> HMSPSPVPGSQNVPAPAVKKISQYACQRRTTLNNYNQLFTDALDILAENDELRENEGSCLAFMRASSVLKSLPFPITSMKDTEGIPCLGDKVKSIIEGIIEDGESSEAKAVLNDERYKSFKLFTSVFGVGLKTAEKWFRMGFRTLSKIQSDKSLRFTQMQKAGFLYYEDLVSCVNRPEAEAVSMLVKEAVVTFLPDALVTMTGGFRRGKMTGHDVDFLITSPEATEDEEQQLLHKVTDFWKQQGLLLYCDILESTFEKFKQPSRKVDALDHFQKCFLILKLDHGRVHSEKSGQQEGKGWKAIRVDLVMCPYDRRAFALLGWTGSRQFERDLRRYATHERKMMLDNHALYDRTKRVFLEAESEE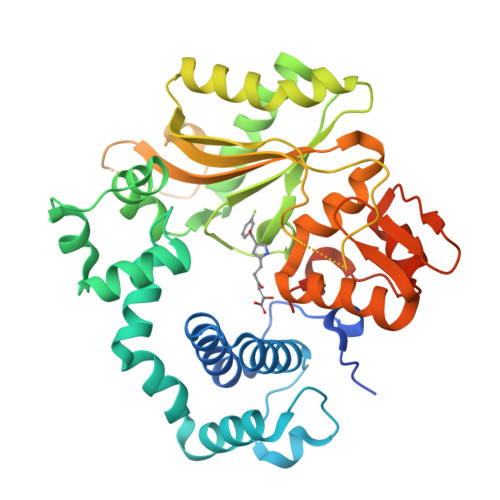EIFAHLGLDYIEPWERNAMGSSHHHHHHSSGLVPRGS4-[(~{Z})-1-cyano-2-[5-[2-(dimethylamino)ethyl-methyl-amino]pyrazin-2-yl]ethenyl]benzenecarbonitrile | C19 H20 N6 | 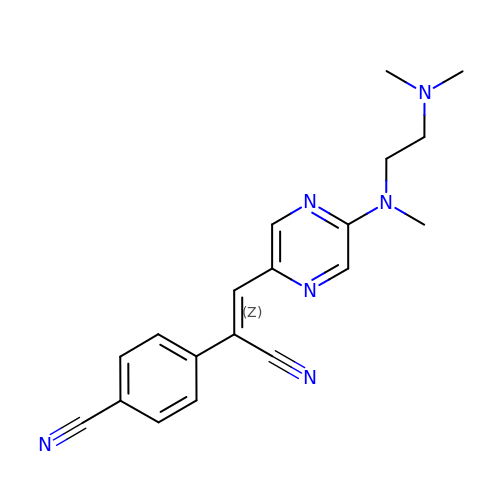LKDZROJVPDPWQB-LICLKQGHSA-N> MVMEYLVLEKRLKRLREVLEKRQKDLIVFADNVKNEHNFSAIVRTCDAVGVLYLYYYHAEGKKAKINEGITQGSHKWVFIEKVDNPVQKLLEFKNRGFQIVATWLSKESVNFREVDYTKPTVLVVGNELQGVSPEIVEIADKKIVIPMYGMAQSLNVSVATGIILYEAQRQREEKGMYS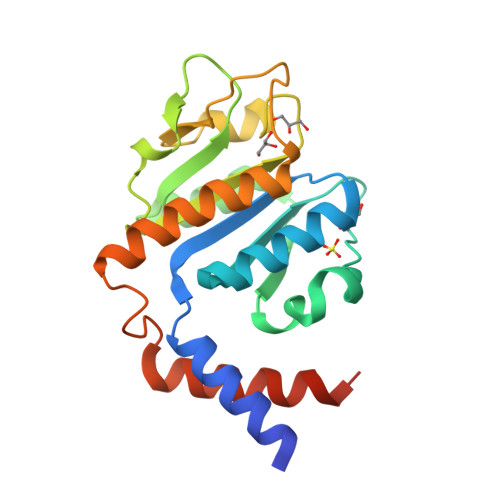RPSLSEEEIQKILKKWAYEDVIKERKRTLSTS> AGWNVNSKQNIAVYWGQNSANSQSTQQRLSFYCNDANINVIDIAFLNGITPPMTNFANAGDRCTPFSDNPWLLQCPEIEADIKTCQANGKTILLSLGGDSYTQGGWSSTGAAQSAADQVWAMFGPVQSGSSVHRPFGSAVVDGFDFDFEATTNNLAAFGAQLKSRTNAAGGKKYYFSAAPQCFFPDAAVGALINAVPMDWIQIQFYNNPCGVSGFTPGTSTQNNYNYQTWENWAKTSPNPNVKLLVGIPAGPGAGRGYVSGSQLTSVFQYSKGFST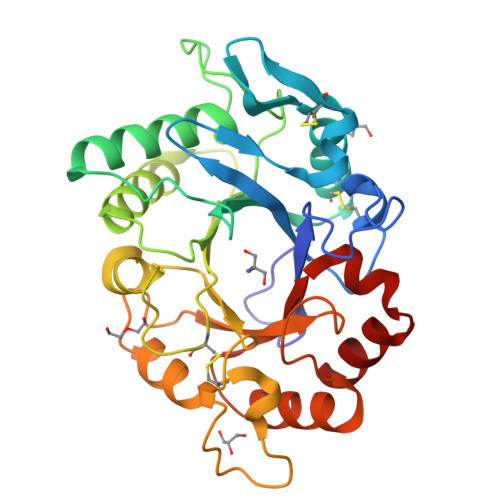FAGAMMWDMSQLYQNTGFETQVVNALR>[2x]MSTGDSFETRFEKMDNLLRDPKSEVNSDCLLDGLDALVYDLDFPALRKNKNIDNFLSRYKDTINKIRDLRMKAEDYEVVKVIGRGAFGEVQLVRHKSTRKVYAMKLLSKFEMIKRSDSAFFWEERDIMAFANSPWVVQLFYAFQDDRYLYMVMEYMPGGD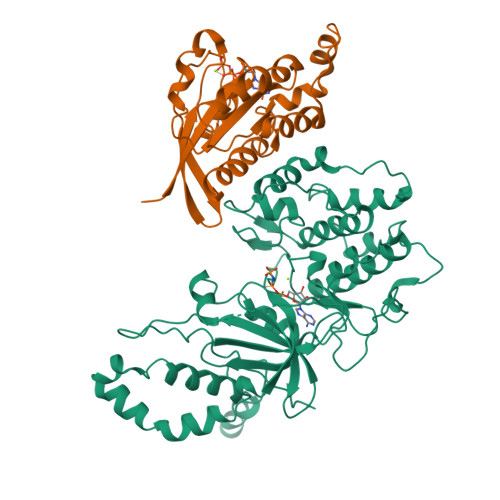LVNLMSNYDVPEKWARFYTAEVVLALDAIHSMGFIHRDVKPDNMLLDKSGHLKLADFGTCMKMNKEGMVRCDTAVGTPDYISPEVLKSQGGDGYYGRECDWWSVGVFLYEMLVGDTPFYADSLVGTYSKIMNHKNSLTFPDDNDISKEAKNLICAFLTDREVRLGRNGVEEIKRHLFFKNDQWAWETLRDTVAPVVPDLSSDIDTSNFDDLEEDKGEEETFPIPKAFVGNQLPFVGFTYYSNRRYL;>MKERRASQKLSSKSIMDPNQNVKCKIVVVGDSQCGKTALLHVFAKDCFPENYVPTVFENYTASFEIDTQRIELSLWDTSGSPYYDNVRPLSYPDSDAVLICFDISRPETLDSVLKKWKGEIQEFCPNTKMLLVGCKSDLRTDVSTLVELSNHRQTPVSYDQGANMAKQIGAATYIECSALQSENSVRDIFHVATLACVNK[2x]RexA and RexB function as an exclusion system that prevents bacteriophage T4rII mutants from growing on Escherichia coli λ phage lysogens. Recent data established that RexA is a non-specific DNA binding protein that can act independently of RexB to bias the λ bistable switch toward the lytic state, preventing conversion back to lysogeny. The rex genes are situated directly adjacent the cI repressor gene in the λ genome and are transcribed from the same PRM maintenance promoter that drives constitutive expression of the repressor during lysogeny. They produce a 31 kDa soluble protein, RexA, and a 16 kDa protein, RexB. Here, we have shown by X-ray crystallography that the λ RexA protein has a split, two-domain architecture that shares structural homology with RdgC.

The resulting structure, however, was incomplete and was thus used as a search model for molecular replacement to solve crystal form 2, which refined to 2.05-Å resolution with an Rwork/Rfree of 20.6%/25.1%. The final model shows a symmetric dimer that measures 95 Å along the longest axis. Each monomer contains a split globular domain (residues 1–139 and 248–279) comprised of a seven-stranded antiparallel β-sheet flanked by α-helices that is divided by a dimerization domain consisting of a four-stranded antiparallel β-sheet with four α-helices localized on one face (residues 143–234). These domains are connected via two flexible linkers that we term the hinge loop and the swivel loop (235–247). The β-sheets of the dimerization domain pack together to form a continuous eight-stranded anti-parallel platform above which helices α6, α7 and η1 interdigitate. The globular domains are situated below the dimerization domains and have only minimal contact across the 2-fold symmetry axis via the C-terminus of the α8 helix. This helix kinks at residues 261–263 and interacts with strand β11 of its affiliated dimerization domain, anchored by a salt bridge between D215 and R261. A bound sulfate and two cadmium ions from the crystallization solution provide further hydrogen bonding contacts in this region in monomer A. The sandwiching of a cadmium ion between two monomers at the two-fold symmetry axis produced a significant change in packing relative to crystal form 1, which ultimately yielded the high-resolution diffraction. Superposition of RexA and RdgC shows that the orientation of the globular domains in the crystallized RexA dimer occludes the space beneath the dimerization interface, blocking the formation of an analogous pore and preventing DNA from associating in the same manner. Based on this modeling, we predict RexA undergoes a major conformational change that reorients the globular domains to facilitate DNA binding.

>[2x]MKNGFYATYRSKNKGKDKRSINLSVFLNSLLADNHHLQVGSNYLYIHKIDGKTFLFTKTNDKSLVQKINRSKASVEDIKNSLADDESLGFPSFLFVEGDTIGFARTVFGPTTSDLTDFLIGKGMSLSSGERVQIEPLMRGTTKDDVMHMHFIGRTTVKVEAKLPVFGDILKVLGATDIEGELFDSLDIVIKPKFKRDIKKVAKDIIFNPSPQFSDISLRAKDEAGDILTEHYLSEKGHLSAPLNKVTNAEIAEEMAYCYARMKSDILECFKRQVGKVKD>MKVVDISKINELVKEGATLMIGGFLGVGTPENIIDEIIRHNISNLTVIANDTAFEDRGIGKLVKNKLCKKVIVSHIGTNPETQRQMIEGTLEVELVPQGTLAERIRAAGVGLGGILTPTGVGTVVEKDKKVIEVEGKKYLLELPIHADVALIKAKKADYLGNLVYNLTAENFNPIMALAAKTVIAEVEEIVPTGTLSPNEIKTPGIIVDYIVTGVTR[2x];>MNPKEKIAIRVAQELKKGQLVNLGIGLPTLVANYIPKDIHVFFQSDNGIIGMGPAPKEGYENSDLTNAGASYITALPGAMTFDSAFSFGIIRGGHLDVTVLGGLQVDEEGHLANWMIPGKMIPGMGGAMDLVTGAKKVIVAMTHTAKGTPKIVKKCTLPLTSIRKVDLIVTELAVIEPTDEGLLLKEISKETTLDEVLKLTEAKLIIADDLKIFA[2x]

CtfAB then transfers the CoA from acetoacetyl-CoA to acetate to reform an acetyl-CoA and produce acetoacetate. CtfAB is a member of family 1 CoA transferases. CtfB contains the acetyl-CoA binding site and the PS01724 signature sequence which includes the catalytic glutamate residue (E46) sandwiched between two short antiparallel beta strands on the N-terminal end of an eight-stranded mixed beta sheet. CtfA contains the acetate binding site and the PS01723 signature sequence.

Based on previous reports, mutation of the catalytic residue on the beta subunit (residue 46) from a glutamate to aspartate (βE46D) should convert the CoA transferase into a CoA hydrolase. Here, creation of the E46D mutant in the B subunit converted the transferase into a hydrolase, with activity confirmed on acetoacetyl-CoA. Evaluation using the in vitro acetone pathway assay at 70°C showed that, in contrast with the WT enzyme, activity of the E46D mutant did not require acetate; acetone formation was the same at 150 mM or 0 mM potassium acetate (0.2–0.3 mM produced from 5 mM acetyl-CoA). In other CtfAB, mutation of the catalytic glutamate to aspartate creates an enzyme that is unable to form covalent aspartyl adducts but is competent for hydrolase activity. A proposed mechanism for the hydrolase activity involves the aspartate carboxylate acting as a general base to activate a water molecule for nucleophilic attack. The E46D mutant is partially active as a hydrolase but cannot catalyze the CoA transferase reaction. In contrast, the shorter D46 does not reach into the acetate binding pocket and instead is rotated away from the acetate binding pocket and positioned to form a hydrogen bond with the side chain nitrogen of N22. The catalytic glutamate is closer, more flexible, and better positioned for direct attack, whereas the aspartate residue is less flexible and partially fixed further away from the active site by the hydrogen bond with N22 making direct attack unlikely, but E46D could activate a water molecule and position it for nucleophilic attack. Based on previous literature, this is the first structural evidence from substrate bound crystal structures that supports the proposed mechanism for how the E46D mutation converts the CoA transferase into a CoA hydrolase 28. Attempts to convert T. mel CtfAB into a hydrolase (β, E46D mutation) worked but was too promiscuous to be useful for specific use in the acetone production pathway.> MNFIRNNRRALIQRMGLTVTKQICDDLFALNVLNNQEANVIYCEPLEQEAARKIIHMTMQKGSAACNLFLKSLENWDYFVYQDLTGQNLSYQVTEEDLNVLAQNLKDLYNSPAFLNFYPLGEDIDIIFNLEKTFTEPIMWKKDHRHHRVEQLTLGSLLEALKSPCLIEGESGKGKSTLLQRIAMLWASGGCRALKGFRLVFFIHLRSARGGLFETLYDQLLNIPDFISKPTFKALLLKLHKEVLFLLDGYNEFHPQNCPEIEALIKENHRFKNMVIVTTTTECLRHIRHVGALTAEVGDMTEDSAKDLIEAVLVPDQVERLWAQIQESRCLRNLMKTPLFVVITCAIQMGRQEFQAHTQTMLFQTFYDLLIQKNSHRYRGGASGDFARSLDYCGDLALEGVFAHKFDFEPEHGSSMNEDVLVTIG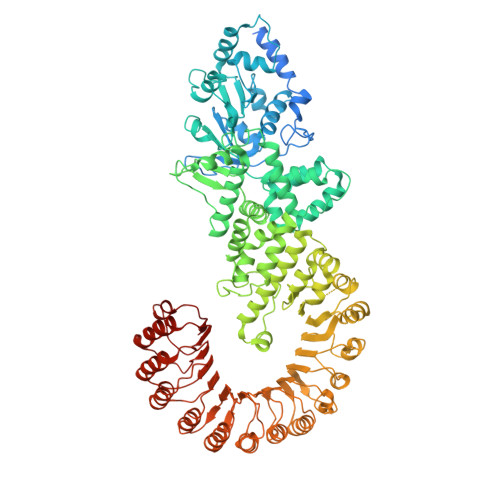LLCKYTAQRLKPTYKFFHKSFQEYTAGRRLSSLLTSKEPEEVSKGNSYLNKMVSISDITSLYGNLLLYTCGSSTEATRAVMRHLAMVYQHGSLQGLSVTKRPLWRQESIQSLRNTTEQDVLKAINVNSFVECGINLFSESMSKSDLSQEFEAFFQGKSLYINSENIPDYLFDFFEYLPNCASALDFVKLDFYERATESQDKAEENVPGVHTEGPSETYIPPRAVSLFFNWKQEFKTLEVTLRDINKLNKQDIKYLGKIFSSATNLRLHIKRCAAMAGRLSSVLRTCKNMHTLMVEASPLTTDDEQYITSVTGLQNLSIHRLHTQQLPGGLIDSLGNLKNLERLILDDIRMNEEDAKNLAEGLRSLKKMRLLHLTHLSDIGEGMDYIVKSLSEESCDLQEMKLVACCLTANSVKVLAQNLHNLIKLSILDISENYLEKDGNEALQELIGRLGVLGELTTLMLPWCWDVHTSLPKLLKQLEGTPGLAKLGLKNWRLRDEEIKSLGEFLEMNPLRDLQQLDLAGHCVSSDGWLYFMNVFENLKQLVFFDFSTEEFLPDAALVRKLSQVLSKLTLLQEVKLTGWEFDDYDISAIKGTFKLVTA>[2x]MKFKWDEFFVTGDPLILGAQVSIALSTIAIIFVLTYFKKWKWLWSEWITTVDHKKLGIMYIISAVIMLFRGGVDGLMMRAQLALPNNSFLDSNHYNEIFTTHGTIMIIFMAMPFLIGLINVVVPLQIGARDVAFPYLNNLSFWTFFVGAMLFNISFVIGGSPNAGWTSYMPLASNDMSPGPGENYYLLGLQIAGIGTLMTGINFMVTILKMRTKGMTLMRMPMFTWTTLITMVIIVFAFPVLTVALALLSFDRLFGAHFFTLEAGGMPMLWANLFWIWGHPEVYIVILPAFGIFSEIISSFARKQLFGYKAMVGSIIAISVLSFLVWTHHFFTMGNSASVNSFFSITTMAISIPTGVKIFNWLFTMYKGRISFTTPMLWALAFIPNFVIGGVTGVMLAMAAADYQYHNTYFLVSHFHYVLIAGTVFACFAGFIFWYPKMFGHKLNERIGKWFFWIFMIGFNICFFPQYFLGLQGMPRRIYTYGPNDGWTTLNFISTVGAFMMGVGFLILCYNIYYSFRYSTREISGDSWGVGRTLDWATSSAIPPHYNFAVLPEVKSQDAFLHMKEEKTELYPESKFKKIHMPSNSGRPFFMSVAFGLAGFGLVFEWYWMGVVGLIGVLLCMVLRSFEYDNGYYISVDEIKETERKISE;>[2x]CSNASVLDPKGPVAEQQSDLILLSIGFMLFIVGVVFVLFTIILVKYRDRKGKDNGSYNPEIHGNTFLEVVWTVIPILIVIALSVPTVQTIYSLEKAPEATKDKEPLVVYATSVDWKWVFSYPEQDIETVNYLNIPVDRPILFKISSADSMASLWIPQLGGQKYAMAGMLMDQYLQADKVGTYEGRNANFTGEHFADQEFDVNAVTEKDFNSWVKKTQNEAPKLTKEKYDELMLPENVDELTFSSTHLKYVDHGQ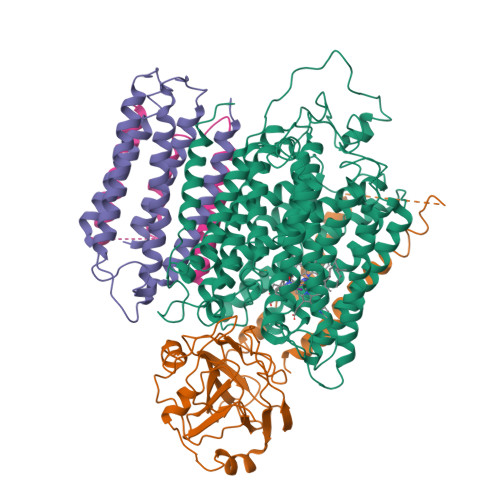DAEYAMEARKRLGYQAVSPHSKTDPFENVKKNEFKKSDDTEE;>MEHAEHGNSNAPMEYQSETGRLNILGFWIFLGAEIVLFSTLFATFFVLKNRTAGGVLPDELFEVNLVMIMTFLLLISSFTCGIAVHEMRRGSLKGVVIWTIITLLLGAGFVGCEINEFVHYVHEGAALSTSAFWSGFFVLLGTHGTHVTIGIFWITGILIQLKKRGLTPQTSSKIFISSLYWHFLDVVWIFIFTGVYLMGLGGL[2x]>[2x]SNAMETSVIEASSLKLD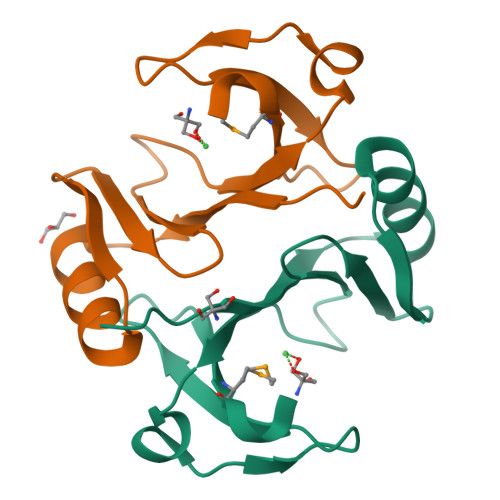DLHHIAISVTDVAQSVEWYTSHFQCRIAYQDSTWALLKFGNLSLALVIPEQHPPHIAFTSDRAGEYGSLKTHRDGTRSCYIQDPSGNSVELMDPTSL> QQYKTFMGARVLWPPEAADDI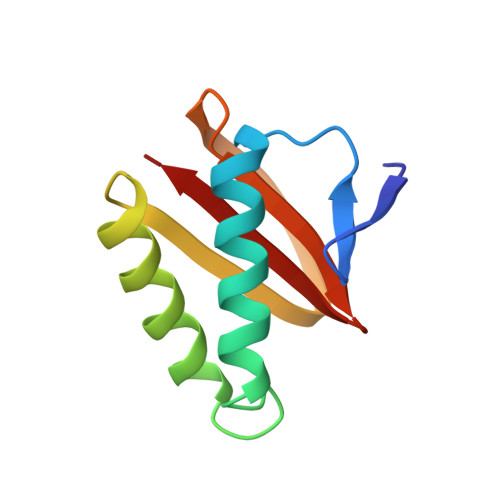LEGAIRETQDALKKFEIAREGQKIAEHLKKYMDDHFDPYWHVFFGKNFGCQAVHNKNRFIYFYIEKTAFLMYQT>[2x]MSSQYIMSTKDGKMITSDSKPKLDKTTGMYLYYD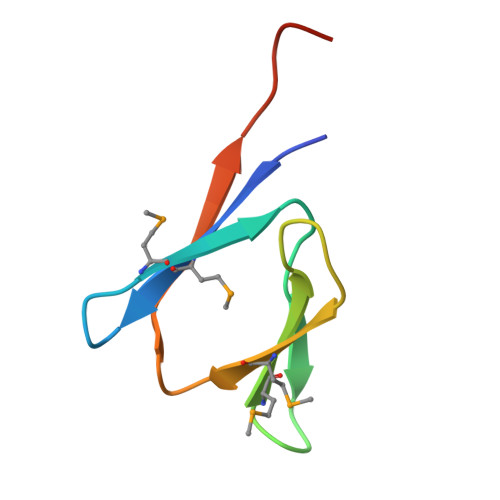EDGREVMIKQEDVTQIIERLEHHHHHH>[2x]VMKALILAGGSGERFWPLSTPETPKQFLKLFGNKSLMRWTFERVLEEMDPKDVIVVTHKDYVERTKKELPELPDENIIAEPMKKNTAPACFIGTKLADDDEPVLVLPADHRIPDTKKFWKTVKKALDALEKYDGLFTFGIVPTRPETGYGYIEIGEELEEGVHKVAQF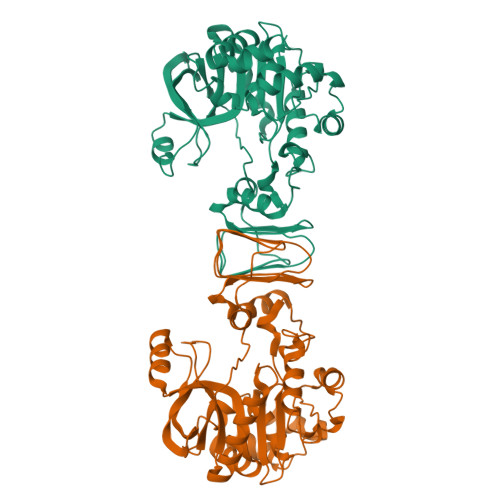REKPDLETAKKFVESGRFLWNSGMFLWKAREFIEEVKVCEPSIYENLKDVDPRNFEELKKAYEKVPSISVDYAVMEKSKKVRVVKADFEWSDLGNWSSVREIEGYTEESDEVILVDSDRVFVKTHNKPIAVVGLSDVIVIDTPNGILICKEEYAQKVREVVKKLFRTS> GPMSEAADVERVYAAMEEAAGLLGVACARDKIYPLLSTFQDTLVEGGSVVWFSMASGRHSTELDFSISVPTSHGDPYATVVEKGLFPATGHPVDDLLADTQ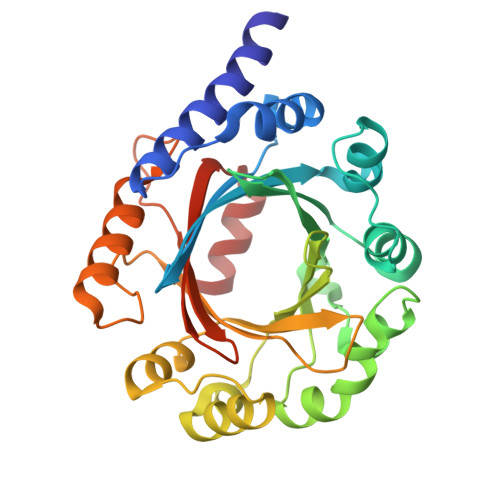KHLPVSMFAIDGEVTGGFKKTYAFFPTDNMPGVAELSAIPSMPPAVAENAELFARYGLDKVQMTSMDYKKRQVNLYFSELSAQTLEAESVLALVRELGLHVPNELGLKFCKRSFSVYPTLNWETGKIDRLCFAVISNDPTLVPSSDEGDIEKFHNYATKAPYAYVGEKRTLVYGLTLSPKEEYYKLGAPYHITDVFRGLLKAFDSLED> LVPRGSHMNTSELRICRINKESGPCTGGEELYLLCDKVQKE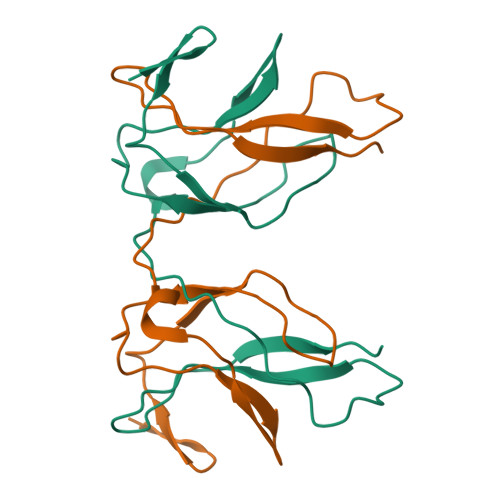DISVVFSTASWEGRADFSQADVHRQIAIVFKTPPYEDLEISEPVTVNVFLQRLTDGVCSEPLPFTYLPR The APOBEC3 family of enzymes (A3A-A3H) forms part of the innate immune response against viruses and transposons. The normally antiviral enzyme APOBEC3A is an endogenous mutagen in human cancer. Its single-stranded DNA C-to-U editing activity results in multiple mutagenic outcomes including signature single-base substitution mutations (isolated and clustered), DNA breakage, and larger-scale chromosomal aberrations. Here, we use X-ray crystallography to determine high-resolution structures of wildtype A3A/hairpin-inhibited complexes and demonstrate the underlying mechanism of inhibition.

All structures exhibit a similar crystal packing and a common tertiary structure for the protein (with minor changes on absence of Zn2+). Surprisingly, they also share very similar conformation of the hairpin loop region’s TT(C/FdZ)G moiety. In all instances, the C0 and T−1 of TTC-hairpin bind to inactive A3A-E72A identically to the binding of FdZ0 and T−1 in TTFdZ-hairpin to wildtype active A3A. Importantly, these structures explain why 3-nt hairpin loops with TTC (or TTFdZ) are preferred A3A substrates (and inhibitors). Taken together, the hairpin stem bestows restricted conformational flexibility for the A3A-binding loop region of hairpin DNA compared to linear ssDNA, thereby enabling enhanced interactions with A3A loop 1 residues Arg28 and His29.

>[2x]MEASPASGPRHLMDPHIFTSNFNNGIGRHKTYLCYEVERLDNGTSVKMDQHRGFLHNQAKNLLCGFYGRHAALRFLDLVPSLQLDPAQIYRVTWFISWSPCFSWGCAGEVRAFLQENTHVRLRIFAARIYDYDPLYKEALQMLRDAGAQVSIMTYDEFKHCWDTFVDHQGCPFQPWDGLDEHSQALSGRLRAILQNQGN>[4x]GSHMSNPFEEYDGGHVVLTDALGRHSLWPAGIAVPAGWSVRHGTDSREGCLAHIEHHWTDLRPTGPAVERAPAGACVHELFEAQAARAPDAVALLHEADELTYGALNERANRLAHRLVGLGVAPGTLVGVHLERGFDMVVALLAVLKAGGGYTMLDPQFPVERLALSLEDTGAPLLVTSRPLSGRLTGTTTLYVEDEAASDAPAGNLATGVGPEDVACVMFTSGSTGRPKGVMSPHRALTGTYLGQDYAGFGPDEVFLQCSPVSWDAFGLELFGALLFGARCVLQSGQNPDPLEIGELVARHGVTMLQLSASLFNFLVDEVPEAFEGVRYAITGGEPASVPHVAKARRDHPALRLGNGYGPAESMGFTTHHAVVAGDLSGTALPIGVPLAGKRAYVLDDDLKPAANGALGELYVAGAGLAHGYVSRPALTAERFVADPFAGPGGERMYRTGDLARRRADGVLEYVGRADDQVKIRGFRVEPGEV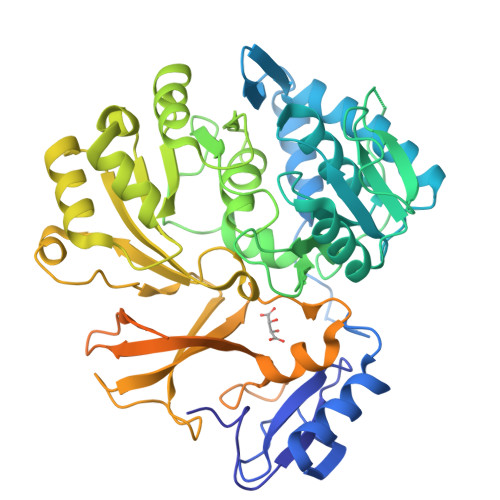EARLVGHPAVRQAAVLAQDSRLGDKQLVAYVVAERADAPPDAAELRRHVAEALPAYMVPVECVPVDELPRTPNGKLDRRALTGSGS>MGSDKIHHHHHHMDRIIEKLDHGWWVVSHEQKLWLPKGELPYGEAANFDLVGQRALQIGEWQGEPVWLVQQQRRHDMGSVRQVIDLDVGLFQLAGRGVQLAEFYRSHKYCGYCGHEMYPSKTEWAMLCSHCRERYYPQIAPCIIVAIRRDDSILLAQHTRHR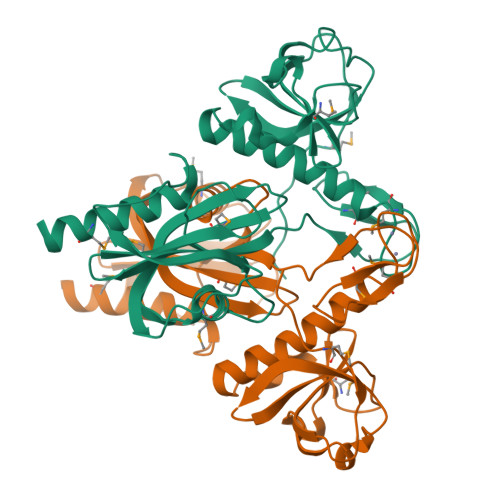NGVHTVLAGFVEVGETLEQAVAREVMEESGIKVKNLRYVTSQPWPFPQSLMTAFMAEYDSGDIVIDPKELLEANWYRYDDLPLLPPPGTVARRLIEDTVAMCRAEYE[2x]> MR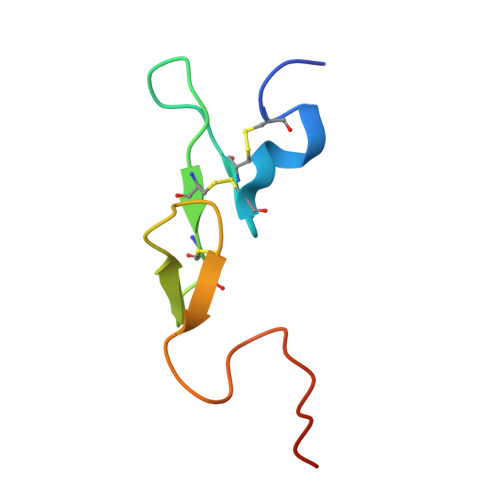KLCSLDNGDCDQFCHEEQNSVVCSCARGYTLADNGKACIPTGPYPCGKQTLERRKR5-fluoro-3-methyl-2-{4-[4-(trifluoromethoxy)benzyl]phenyl}quinolin-4(1H)-one 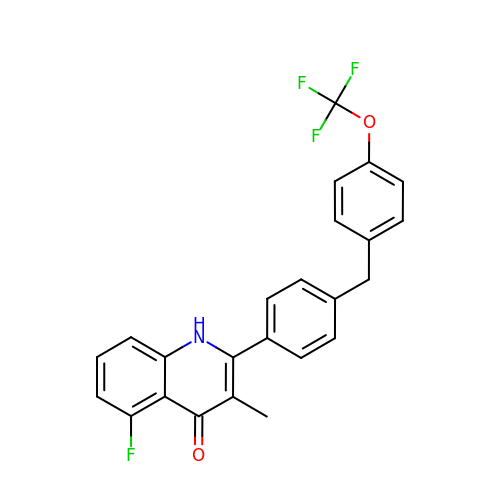| C24 H17 F4 N O2 | OPUNZJHITPCTFC-UHFFFAOYSA-N>[10x]MEGLNLVATALAVGLGAIGPGVGIGIIVSGAVQAIGRNPEIENRVVTYMFIGIAFTEALAIFGLVIAFLIGFGVLQ;>MSTRTRNILIIVGALIISIASRFFLYTGPPHVEVAAEVIFDGIPGFPITNSFVVAIIIDIFVIALAVAATRNLQMVPRGLQNVMEFILESLYNLFRNINAKYVATAFPLVATIFLFVLFGNWFGLLPGVGSIGVCHEKKEEHAVVDERLALAAPAAPLSSVAAAEGEEIHDTCAAQGKKLVPLFRAPAADLNFTFAIAVISFVFIEYWGFRALGPGYLKKFFNTNGIMSFVGIIEFISELVKPFALAFRLFGNIFAGEVLLVVMAFLVPLLLPLPFYGFEVFVGFIQALIFALLTYAFLN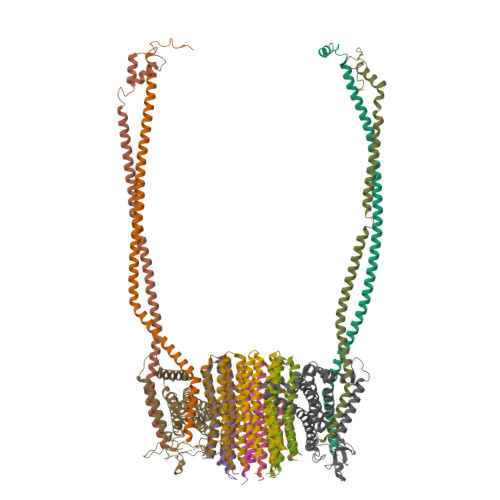IAVTGHDEEHAH[2x];>MEALGINPTLFIAQLINFLLLIFILRALLYRPVMNLLNERTRRIEESVRDAEKVREQLANARRDYEAEIARARQEAAKIVAQAQERAKQQEAEIIAQARREAERLKEEARAQAEQERIRMLSEAKSQIADLVTLTASRVLGAELQARGHDALIAESLAALDRRN[4x]> MNHKVHHHHHHIEGRHMASAGDVTRAALPRAQPRAEGPACVLGIGTAVPPAEFLQSEYPDFFFNITNCGEKEALKAKFKRICDKSGIRKRHMFLTEEVLKANPGICTYMEPSLNVRHDIVVVQVPKLAAEAAQKAIKEWGGRKSDITHIVFATTSGVNMPGADHALAKLLGLKPTVKRVMMYQTGCFGGASVLRVAKDLAENNKGARVLAVASEVTAVTYRAPSENHLDGLVGSALFGD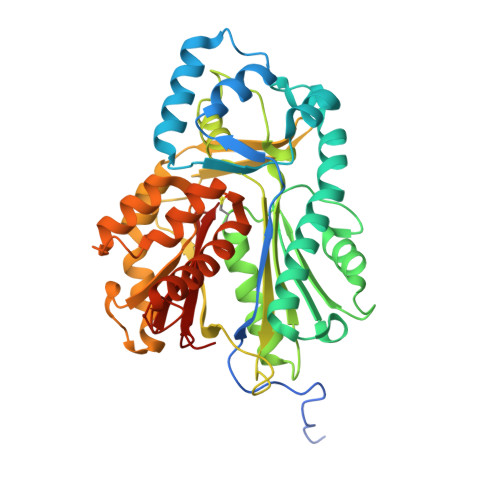GAGVYVVGSDPKPEVEKPLFEVHWAGETILPESDGAIDGHLTEAGLIFHLMKDVPGLISKNIEKFLNEARKPVGSPAWNEMFWAVHPGGPAILDQVEAKLKLTKDKMQGSRDILSEFGNMSSASVLFVLDQIRHRSVKMGASTLGEGSEFGFFIGFGPGLTLEVLVLRAAPNSA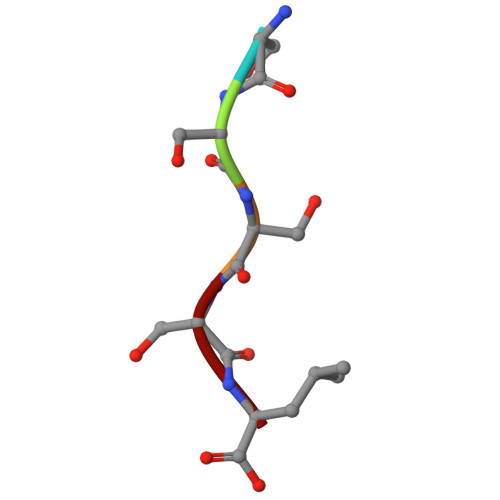> SSSSL>MAASLPSTLSFSSAPDEIQHPQIKFSEWKFKLFRVRSFEKAPEEAQKEKDSSEGKPYLEQSPVVPEKPGGQNSILTQRALKLHPKFSKKFHADGKSSDKAVHQARLRHFCRICGNRFKSDGHSRRYPVHGPVDAKTQSLFRKKEKRVTSWPDLIARIFRIDVKADVDSIHPTEFCHDCWSIMHRKFSSSHSQVYFPRKVTVEWHPHTPSCDICFTAHRGLKRKRHQPNVQLSKKLKTVLNHARRDRRKRTQARVSSKEVLKKISNCSKIHLSTKLLAVDFPAHFVKSISCQICEHILADPVETSCKHLFCRICILRCLKVMGSYCPSCRYPCFPTDLESPVKSFLNILNSLMVKCPAQDCNEEVSLEKYNHHVSSHKESKETLVHINKGGRPRQHLLSLTRRAQKHRLRELKIQVKEFADKEEGGDVKAVCLTLFLLALRARNEHRQADELEAIMQGRGSGLQPAVCLAIRVNTFLSCSQYHKMYRTVKAITGRQIFQPLHALRNAEKVLLPGYHPFEWQPPLKNVSSRTDVGIIDGLSGLASSVDEYPVDTIAKRFRYDSALVSALMDMEEDILEGMRSQDLDDYLNGPFTVVVKESCDGMGDVSEKHGSGPAVPEKAVRFSFTVMRITIEHGSQNVKVFEEPKPNSELCCKPLCLMLADESDHETLTAILSPLIAEREAMKSSELTLEMGGIPRTFKFIFRGTGYDEKLVREVEGLEASGSVYICTLCDTTRLEASQNLVFHSITRSHAENLQRYEVWRSNPYHESVEELRDRVKGVSAKPFIETVPSIDALHCDIGNAAEFYKIFQLEIGEVYKHPNASKEERKRWQATLDKHLRKRMNLKPIMRMNGNFARKLMTQETVDAVCELIPSEERHEALRELMDLYLKMKPVWRSSCPAKECPESLCQYSFNSQRFAELLSTKFKYRYEGKITNYFHKTLAHVPEIIERDGSIGAWASEGNQSGNKLFRRFRKMNARQSKCYEMEDVLKHHWLYTSKYLQKFMNAHNALKSSGFTMNSKETLGDPLGIEDSLESQDSMEF[2x];>[2x]MSLQMVTVGHNIALIQPGFSLM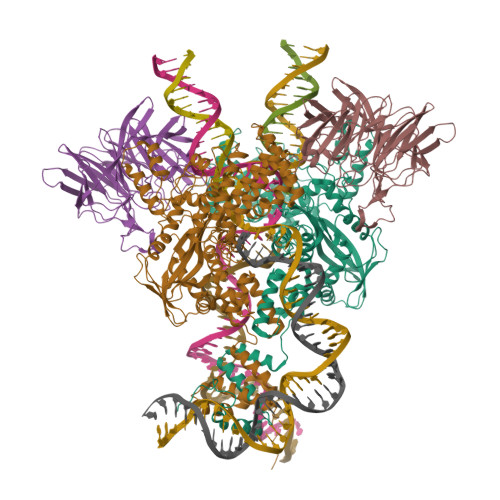NFDGQVFFFGQKGWPKRSCPTGVFHFDIKQNHLKLKPAIFSKDSCYLPPLRYPATCSYKGSIDSDKHQYIIHGGKTPNNELSDKIYIMSVACKNNKKVTFRCTEKDLVGDVPEPRYGHSIDVVYSRGKSMGVLFGGRSYMPSTQRTTEKWNSVADCLPHVFLIDFEFGCATSYILPELQDGLSFHVSIARNDTVYILGGHSLASNIRPANLYRIRVDLPLGTPAVNCTVLPGGISVSSAILTQTNNDEFVIVGGYQLENQKRMVCSLVSLGDNTIEISEMETPDWTSDIKHSKIWFGSNMGNGTIFLGIPGDNKQAMSEAFYFYTLRCSEEDLSEDQKIVSNSQTSTEDPGDSTPFEDSEEFCFSAEATSFDGDDEFDTYNEDDEDDESVTGYWITCCPTCDVDINTWVPFYSTELNKPAMIYCSHGDGHWVHAQCMDLEERTLIHLSEGSNKYYCNEHVQIARALQTPKRNPPLQKPPMKSLHKKGSGKVLTPAKKSFLRRLFD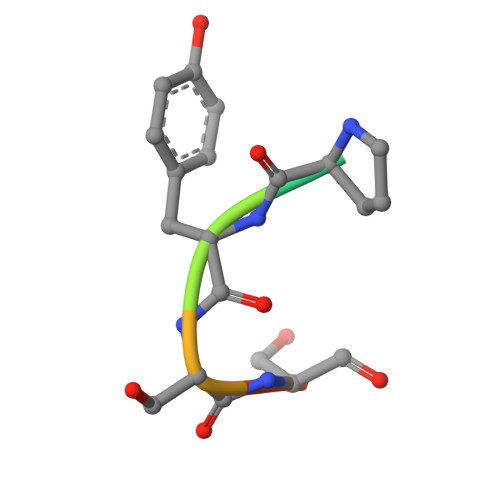> VPYSSAQ> SGEIRPTIGQQMETGDQRFGDLVFRQLAPNVWQHTSYLDMPGFGAVASNGLIVRDGGRVLVVDTAWTDDQTAQILNWIKQEINLPVALAVVTHAHQDKMGGMDALHAAGIATYANALSNQLAPQEGMVAAQHSLTFAANGWVEPATAPNFGPLKVFYPGPGHTSDNITVGIDGTDIAFGGCLIKDSKAKSLGNLGDADTEHYAASARAFGAAFPKASMIVMSHSAPDSRAAITHTARMADKLR

As one of the resistance determinants, metallo-β-lactamases (MBLs), including imipenemases (IMPs), Verona integron-encoded metallo-β-lactamases (VIMs), and more recent New Delhi metallo-β-lactamases (NDMs), are Zn(II)-containing enzymes that activate a nucleophilic water to cleave the β-lactam ring, conferring onto bacteria the resistance to the last resort carbapenems and all other bicyclic β-lactams that are currently used. In particular, NDM-1 is one of the most widespread and threatening MBLs that binds and hydrolyzes almost all β-lactam antibiotics with Zn(II) as a cofactor. Moreover, the active site of NDM-1 is located in a shallow groove encompassed by several loops with Zn(II) coordinating residues, which confers conformational flexibility of these residues for efficient substrate binding and catalysis turnover. Crystallographic and biophysical studies demonstrate that Bi(III) compounds irreversibly inactivate NDM-1 by a unique mechanism, with one Bi(III) replacing two zinc ions in the active site.

We first crystallized and determined the high-resolution native NDM-1 structure at 0.95 Å, the highest resolution obtained so far. No significant overall conformational changes were observed between the Bi-bound and Zn-bound NDM-1 (rmsd of 0.18 Å over all Ca), while only subtle conformational changes were observed at the active site.> MKLTDGQIRINHVSSEKKRRELERAIFDEL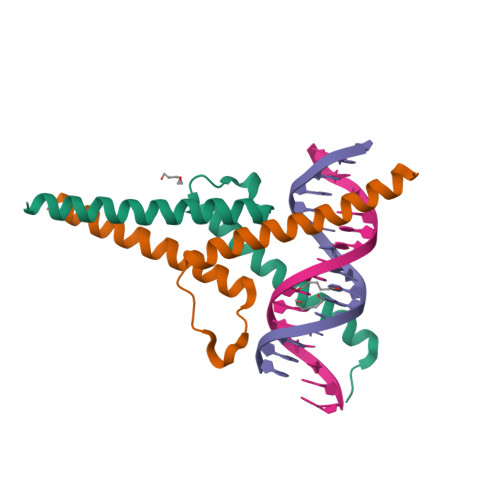VAVVPDLQPQESRSELIIYLKSLSYLSWLYERNEKLRKQIIAKHE;> DDPVKVRKWKHVQMEKIRRINTKEAFERLIKSVRTPPKENGKRIPKHILLTCVMNDIKSIRSANEALQHILDD In this study we report the enzymatic characterization and the atomic structure of NopAA, which is the first high resolution structure of a rhizobial T3E. The N-terminal end of NopAA contains Type III secretion signals and the C-terminal domain of NopAA has been classified in glycoside hydrolase family 12 (GH12) of the CAZY database. Obtained results showed that NopAA has a xyloglucanase activity that may play a role in cell wall disruption facilitating effector translocation. NopAA as all T3Es possesses a secretion region at its N-terminus.

We obtained unique crystals of the truncated effector NopAAΔ48 from Sinorhizobium fredii USDA257 in complex with cellobiose, diffracting to 2.2 Å resolution. Crystals contain 53% of solvent and four molecules (molecule A, B, C, D) per asymmetric unit covering the entire NopAAΔ48 chain (except molecule B). NopAAΔ48 adopts a β-jelly roll fold typical of enzymes of family GH1224 with a large substrate binding cleft, containing substrate binding subsites running across the surface of the enzyme. In NopAA, these conserved residues are Glu117 (nucleophile) and Glu216 (acid/base residue). The electron density shows sugar units in the positive subsites of the molecules D and A of the asymmetric unit: two glucose moieties of the product cellobiose in molecule D (subsites +1 and +2) and one moiety (subsite +1) in molecule A could be refined in the crystal structure with an occupancy of 0.3. The cellobiose binds to subsites +1 and +2 making few interactions with the enzyme, which is consistent with the fact that cellobiose is the leaving group of the reaction and probably has low affinity for the enzyme. In molecules A and D, the glucose moiety bound in the +1 subsite interacts through its O3 and O4 hydroxyl groups with OE1 and OE2 of Glu216 (the acid/base catalytic residue). In molecule B which is not in complex with cellobiose, the residues 141–146 of the long β9/β10 loop are not defined in the electron density map whereas in molecules D and A, this region is stabilized by the interaction with cellobiose. The β9/β10 loop, close to positive subsites is very dynamic in the free enzyme and probably prevents crystallization of NopAAΔ48 in the absence of cellobiose. NopAA possesses a specific insertion loop between β9 and β10 longer (25 residues, from 125 to 154) than the equivalent loops in the other xyloglucanases (10 amino-acid residues in XEG, and 4 residues in BlXG12).

>[4x]MHHHHHHITSLYKKAGMPIWSSHAPYGSFSRDGYSWNNDVWGPRPGPQTISVSGVNRWSVWSDQPNTPGIKSYPHVAFNIGKPLSSINTLSSSFNQEVPTGGAWDVAYDIWDSSNKHEIMLWTNYTGNSDGSGNVKPISYHYAPSGAAIPVYSNVNVGGATWNVFEGEGPDGHKVISLLRTSKTNSGTVDIKSILQWIKSKGYFGDIEVGSVQYGVEITSSPGGKNFNFNNWSVTSK>MHYAEAATPAKSAGSAVAKKHLEAKQKIGFVHGIDGTIATIAPAASKVTVPYNTVLEIAVSATNIANALVFNLEKDGSIGVILLDNISEVRSGQDVYATGSLLKIPVGFHMLGKIINPLGKEIPTGLFTKAAPLLDDTKLGLVEEMAPNIVSRQPVNYNLLTGYKVIDTLIPVGRGQRELILGDRQTGKTSIALSTILNQTKVNNEILSKNNVLSVYVSIGQRCSNVARIHRLLTEYDAMKYCTIVAATAADPAGLQYLAPYAGTTLGEEFRNSGRHILLVYDDLSKQAVSYRQISLLLRRPPGREAYPGDVFYLHSRLLERSAMMSPQKGSGSLTSLPIVETLSNDVTAYIVTNVISITDGQIYLDAKLFTGGQRPAVNIGLSVSRVGSSAQNKAMKKVGGALKMLMGEYRKMAGEQTSGSQNVSPVMIRGARCLQLFNQKGPSYFMDAIVALYAVTNGYMDDVKLQYSKFYEFLLLNKDLPVLYGQVNNKYFYMYNKNLNYFIRYFGLNHEILEPELKKYIEIHTNLFLDNYQSRMNELKSDEDLVQLKNLLYACKRTV[3x];>[3x]TAPATAADVKQVGYVQQIIGAVVDVTFTDSVPPVLTALTVDAKETGTLLTMEIVQHLDTKTARCICMSSTDMLRLRTPVVNTGSQITVPVGEATLGRIFNVMGDAIDQRGPVKNKVRWPIHRKAPTLAEQSGKDEVLVTGIKVIDLILPYCKGGKIGLFGGAGVGKTVIIMELINNVAKGHGGYSVFAGVGERTREGTDLYLEMMGSKVIDLQGDSKCVLVYGQMNEPPGARARVAQTALTMAEYFRDEAGQDVLLFVDNVFRFTQANSEVSALLGRIPAAVGYQPTLAEDLGMLQERITSTVKGSITSVQAVYVPADDITDPAPATTFSHLDATTVLSRSVAEAGIYPAVEPLECASRIMDPDAIDVNHYNVAMDIVEMLTKYKELQDIIAVLGIDELSEEDKLIVDRARKVAKFMSQPFAVAEVFTGMKGYYVQLEDCVSDFGSLLMGQCDNIPEMAFYMVGGLDSVKEKAAKMAAEAAAMRERARKAAEAK;> MPGGGTIRFWREKLEGYKKYHQIVKTIKMVTLAKYRQTVVRTRVRDQTLRYTRKALDAKTQDDQEVIEKSECLLYVPITTNRGSCGALNTNMVRYLQEVENPKMTIISVGKKALDAMTKVFQDTYRRTILNDMKQAMSFQFAAYVLEHMNTVPWDRAQIVYNRYHGAASQKLAIFNLPKFEDWKQKLEEDSAGDGKIEEDGLLQSLPMKTALGELEETAVEDFYNFHSCLAVLNAVSENELSEYAARIVAVENQLGNITGLMQLADYTYNKTRKELITAELLEIIGTMTAMHAGKKVGLKKTEFWK;> MRASRTLLLSVSRFMRQDPRKFFPDNGFRFFDGPEDSFGDGNIPAQIILTLTRQDEFILKQEPVAAITIRTNEGEMGVLAGHEYTVQQLAPGILEVEYEGGKKDQYVISGGFAHVNDTG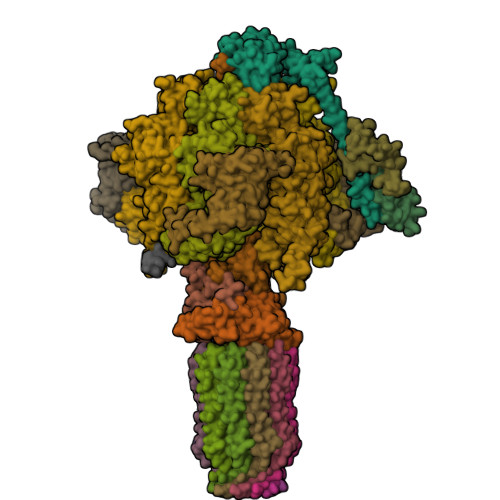VVDINTVEAVPLEEIDHEKLAKALEEARAKSQSPDEAVRIQGEIALEIFEPLEAALH;> MSWRDAGISYLRYLSIVTRCIHEVQKEGPLLTKNVRFSTIGWKSLYLDHGATKEYTAIPAELEKIPENQVAQQHHA;>MQKLSRVVCNRLVRFHGTVAASAGGKRYDLFGYEVSVATGPFIEEIKKAQFYDDAGEVIVKMNLANTPPDLQTYNAVLERILNCKSKRSQPVKGENKFAAMMDILEEMDARSGIKPNAESWGYVLKELVQAGDFRLGWVCIAGMKSLGITPDQALVDANEANAAKAKAAGTDFPAYLKKAAPESFDTKAWGI[3x];> MHMRRAVSVFGRCRSLNGLRNYAVPSPKYIEIYQSDFSRNAYPLELLGGSHVDFAKLLYSFADQVENKKFEVYVEDFKKLDSIIAEKGPFWAEEKIFQSPTFQGLSEGFKFILGWIQSEGAIDRLENVRLAYKELVNEARKETTATVIVAKEPSGNDLAEIRKQVEELHKESPLKDYKLVLETKVDPSIGGGYILEVCNQVVNRSAAAAAAETAALAKASAAQVDWTSLPAAPPRPSPSAPDTLIRLLGSVVDDLADADKVEQKYGA;> MAAACAVRGFTTARPMLTPNKVKVPGRKPQDEEDLTWAEADRKLTPEERYARDKQMALLDKMTSQVEELEKSHTEQKKSNKGVKAQIEAISRQLEALKAQLKE;>[10x]MQRGSSITKVVRRAALARSTRNAAIAYEVTVNGANLIGAGMAASGVGVPAIGVAMCFSSYMLAAARQPNMSAKLLPYCILGFALSEALALFTLLIALLELFVFS;> MFRGFRPVLAADAVKFQTLYNVLTGKQHLKDQVPVKDCNLTAIFGASWKADLNKWFDSEYAPKLPAAERDSAKKSLDLYLKRVDLTRYTREELTTYGILACGPGKVDALTEKHLLETGKARLEELTAGLGNKDEGVNAFRKEVEQEGKYANWPAEKSKALADKVIAASP;> MMRRACRIIRPSHVRGVSGVAPTIYLRSKAALPATSTTDVRPQLYALQRFAKAQLKTATEAERAAIEADIARYQEYLDSDLEKLKQDVAEDTAKKQKLIPLLDRYPDVPIEKIPEHANVLLKKIDACLEILSKDIGEVTDAEAHEMYFETSKFQILHIYTGCVASFPEGDVPPGAVECLPGQVIRTKVNGEDVMLEIDEVDPGYQVCWFKPDVPLPENAEILWSYPYEPTAALPTGTTWEEGQANVLIPAEPTPEAAVWPPTPVTNVYAPMAEKLALKSNPELKVLFKEALLQPAKLLPLDVDYQCSHDREVVEAKRDRYLTALVEAEQAPPLPFTPDVLQLQLEHNVLKGELIDRLRALEYTIVTEQLQARLHERRLRGDVIDEWEELDYHPLVRDDTYLAIDFGDPTFGRYIWKLFPHTDGDEECMFKDTRLDVLPPQVNPLNAILAQHTAQTPVHRSLEKRLWTEVRATAVSE> PNVPSREALAVELSS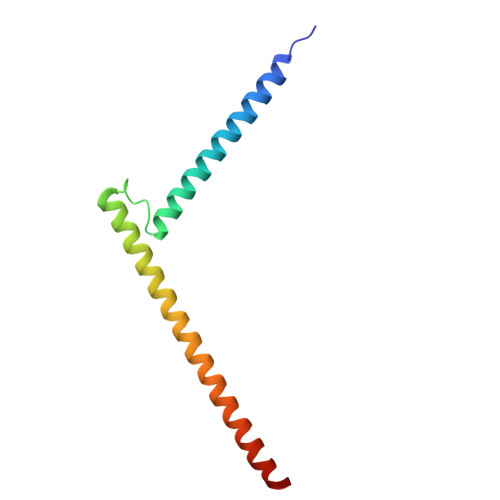QQEYLKLKERYDALQRTQRNLLGEDLGPLSTKELESLERQLDSSLKQIRALRTQFMLDQLNDLQSKERMLTETNKTLRLRLAD>MATTAEILQQVAAGQLSPTAAAQQLEAGKTAALGFANVDLDRQRRNGFPEVIYGAGKTATQIVGIVQALSQQTLPILTTRLSAEKFAALQPALPTAVYHATAQCMTVGEQPAPKTPG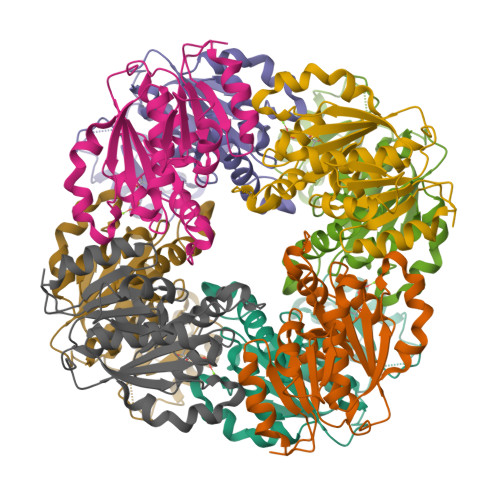YIAVVTAGTSDQPVAEEAAVTAETFGNRVERVYDVGVAGIHRLFAKLDVIRGARVVIVIAGMEGALASVVGGLVDKPVIAVPTSVGYGTSFQGMTALLTMLNSCASGITVVNIDNGFGAAYSASMVNQMASWSHPQFEK[6x]> XYPYSCWVR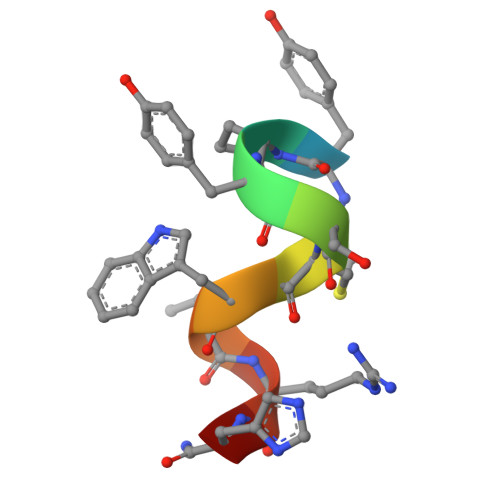HX> GHMDPVQLVNFLQSEHPQTIAVVLSYLDPPVAAQILGALPEELQTEVLKRIALLERTSPEVVKEIERNLEKKISGFVSRTFSKVGGIDTAAEIMNNLDRTTEKKIMDK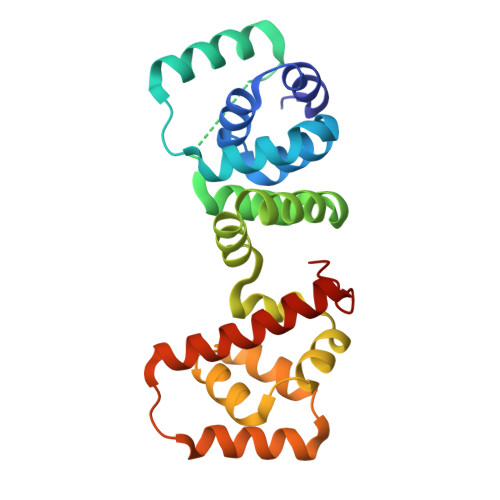LVQENPELADEIRRRMFVFEDILKLDDRSIQLVLREVDTRDLALALKGASDELKEKIFKNMSKRAAALLKDELEYMGPVRLKDVEEAQQKIINIIRRLEEAGEIVIAR>MGSDKIHHHHHHENLYFQGMSKVFVNISLSLDGFMAPEGMDMAHFSDPTYKNWGAKWGALMAWALSQQYLREKLKLGTGGETGPVNDMVRHTFERTGAHIMGKRMFEGGERGWPEEAPFHTPVYVLTHERRNPWVRPGGTTFYFVNDGPEQALALAR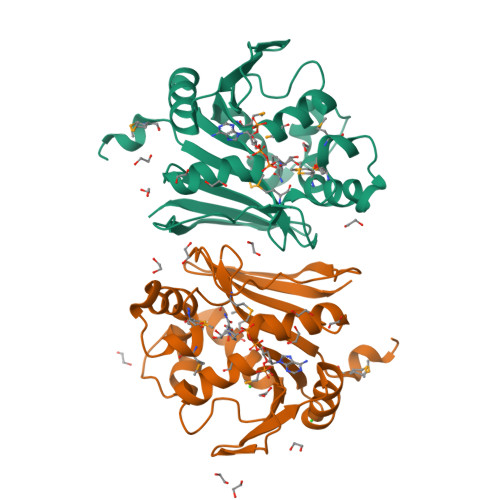EAAGERDIRISGGANVIQQYLNLGLVDELEIALIPVIFGGGRRLFENLHEPLPQFRIDRVLASPTATHLRYVRL[2x]> GGGGGSPEKSPSAQELKEQGNRLFVGRKYP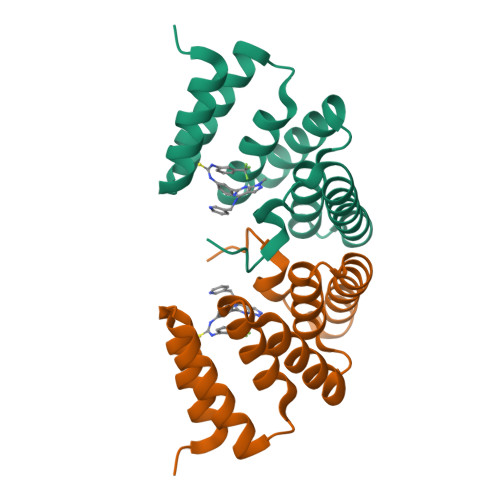EAAACYGRAITRNPLVAVYYTNRALCYLKMQQHEQALADCRRALELDGQSVKAHFFLGQCQLEMESYDEAIANLQRAYSLAKEQRLNFGDDIPSALRIAKKKRWNSIEER> AKLLPPERMKHSIKLVDDQMNWCDSAIEYLLDQTDVLVVGVLGLQGTGKSMVMSLLSANTPEEDQRTYVFRAQSAEMKERGGNQTSGIDFFITQERIVFLDTQPILSPSILDHLINNDRKLPPEYNLPHTYVEMQSLQIAAFLFTVCHVVIVVQDWFTDLSLYRFLQTAEMVK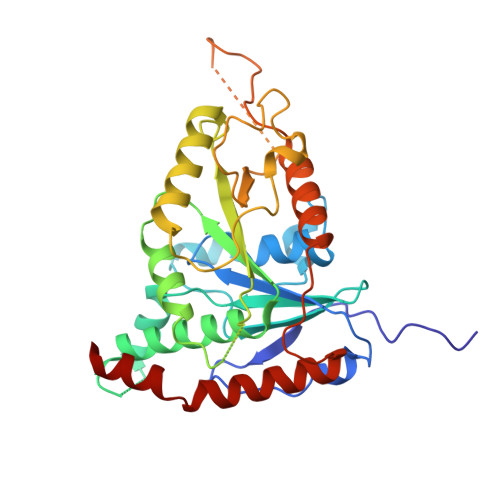PSTPSPSHESSSSSGSDEGTEYYPHLVFLQNKARREDFCPRKLRQMHLMIDQLMAHSHLRYKGTLSMLQCNVFPGLPPDFLDSEVNLFLVPFMDSEAESENPPRAGPGSSPLFSLLPGYRGHPSFQSLVSKLRSQVMSMARPQLSHTILTEKNWFHYAARIWDGVRKSSALAEYSRLLA>MMAGPLSGLRVVELAGIGPGPHAAMILGDLGADVVRIDRPSSVDGISRDAMLRNRRIVTADLKSDQGLELALKLIAKADVLIEGYRPGVTERLGLGPEECAKVNDRLIYARMTGWGQTGPRSQQAGHDINYISLNGILHAIGRGDERPVPPLNLVGDFGGGSMFLLVGILAALWERQSSGKGQVVDAAMVDGSSVLIQMMWAMRATGMWTDTRGANMLDGGAPYYDTYECADGRYVAVGAIEPQFYAAMLAGLGLDAAELPPQNDRARWPELRALLTEAFASHDRDHWGAVFANSDACVTPVLAFGEVHNEPHIIERNTFYEANGGWQPMPAPRFSRTASSQPRPPAATIDIEAVLTDWDGGSGC[2x]

α-Methylacyl-CoA racemase in M. tuberculosis (MCR) has an essential role in fatty acid metabolism and cholesterol utilization, contributing to the bacterium’s survival and persistence. It catalyses the racemization of α-methyl-branched fatty acyl-CoAs, converting the (2S)-epimer to a near racemic mixture of the (2R)- and (2S)-epimers. The enzyme enables the conversion of α-methyl-branched fatty acids derived from cholesterol metabolism into forms that can be utilized by M. tuberculosis for growth and persistence within the host, a key component of M. tuberculosis pathogenesis. Within each active site, the large domain contributes the catalytic residues H126 (part of α-helix 3) and D156 (part of α-helix 5), while the small domain contributes a third catalytic residue, E241 (part of α-helix 9).

Crystals of wild-type MCR formed under a new condition [0.03 M magnesium chloride hexahydrate, 0.03 M calcium chloride dihydrate, 20 % (v/v) ethylene glycol, 10 % (w/v) polyethylene glycol (PEG 8000) and 0.1 M sodium HEPES-MOPS at pH 7.5] after 3 weeks of incubation at 22 °C, and these crystals diffracted to a 1.65 Å resolution and belonged to monoclinic space group C2 with a dimer in the asymmetric unit. The unit cell dimensions for this new crystal form, where a = 181.15 Å, b = 79.16 Å, c = 59.24 Å and β = 91.15˚ and the diffraction resolution cut-off is 1.65 Å, which were selected based on the CC1/2 value and the number of unique reflections present in the structure. The electron density maps for both monomers within the MCR homodimer were of high quality, except for residues 41 to 44, which form part of a flexible loop region. Each monomer (subunit) within the wild-type MCR dimeric structure has a large and a small domain; the large domain consists of residues M1 to A188 and R331 to G360, which come together to form an open α/β sheet structure with a Rossmann-like fold. The small domain has a distinct three-stranded antiparallel β-sheet core structure made up of five α-helices and five β-strands from residues V189 to P300. A surface representation of the MCR structure shows the extended binding groove, which is made up of residues from the large domain of one subunit and the smaller domain of another subunit. Within each active site, the side-chain of D156 sits parallel to H126 (from one monomer), which is hydrogen-bonded to residue E241 from the second monomer. Sandwiched between the D156 and H126 residues, a piece of electron density corresponding to part of a polyethylene glycol molecule (from the crystallization medium) was observed. A network of bound water molecules was also observed within the active site due to the absence of a bound acyl-CoA ester.methyl 2-amino-4-chlorobenzoate | C8 H8 Cl N O2 | 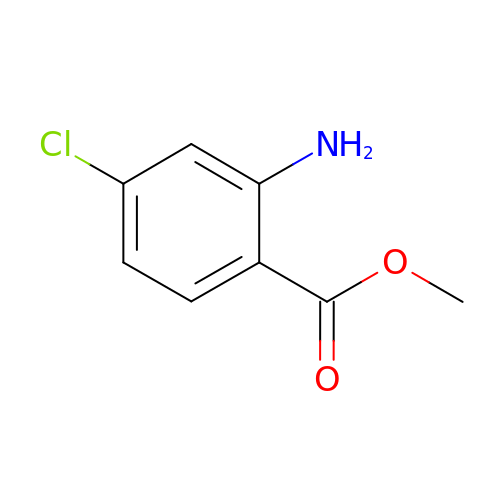YPSSCICDVDOEAI-UHFFFAOYSA-N> ASEMIALNRSLPDVRLEGCKTKVYPDNLPTTSVVIVFHNEAWSTLLRTVHSVINRSPRHMIEEIVLVDDASERDFLKRPLESYVKKLKVPVHVIRMEQRSGLIRARLKGAAVSRGQVITFLDAHCECTAGWLEPLLARIKHDRRTVVCPIIDVISDDTFEYMAGSDMTYGGFNWKLNFRWYPVPQREMDRRKGDRTLPVRTPTMAGGLFSIDRDYFQEIGTYDAGMDIWGGENLEISFRIWQCGGTLEIVTCSHVGHVFRKATPYTFPGGTGQIIN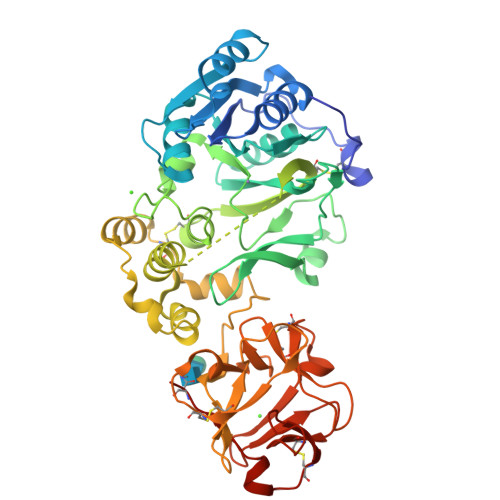KNNRRLAEVWMDEFKNFFYIISPGVTKVDYGDISSRLGLRRKLQCKPFSWYLENIYPDSQIPRHYFSLGEIRNVETNQCLDNMARKENEKVGIFNCHGMGGNQVFSYTANKEIRTDDLCLDVSKLNGPVTMLKCHHLKGNQLWEYDPVKLTLQHVNSNQCLDKATEEDSQVPSIRDCTGSRSQQWLLRNVTLPEIF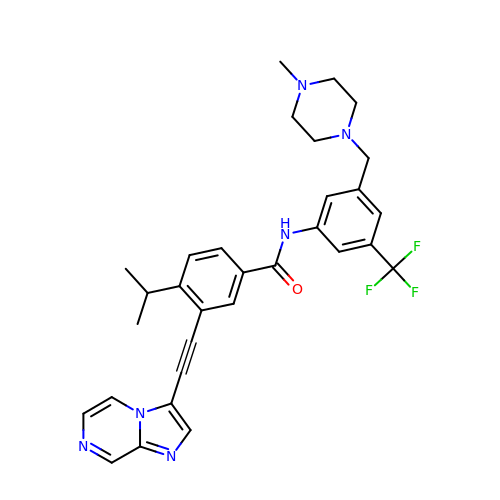3-(2-imidazo[1,2-a]pyrazin-3-ylethynyl)-~{N}-[3-[(4-methylpiperazin-1-yl)methyl]-5-(trifluoromethyl)phenyl]-4-propan-2-yl-benzamide | C31 H31 F3 N6 O | IUGBGEUCXVKGQK-UHFFFAOYSA-N Here, we reveal the extended and contracted atomic structures of an intact contractile-tailed phage (φCD508) that binds to and penetrates the protective S-layer of the Gram-positive human pathogen Clostridioides difficile. The virion can be divided into five distinct regions: the head, neck, tail, baseplate, and needle. Structures of purified φCD508 virions in both extended and contracted conformations were determined by single-particle EM of frozen-hydrated samples; the resolution ranged from 2.6 to 4.0 Å for the extended phage, and 2.9 to 4.2 Å for the contracted form.

The tail is attached to the neck and made up of a stack of 57 nested hexameric tail protein rings, with an inner ring of the tail tube protein gp56 and an outer ring of the tail sheath protein gp55. Each ring is offset from those above and below such that the extended tail assembly can be described as a six-stranded helix, with a twist of 19°, a rise of 39 Å, and an outer diameter of 230 Å. However, a notable feature is that the tail is considerably longer (225 nm) than those of other phages whose structures have been described. In the extended state (left), the sheath forms extensive interactions between the sheath and the tail tube. The main tail tube protein, gp56, has the conserved fold seen in other Caudoviricetes tail tubes. However, gp56 lacks both the ɑ-loop and the N-loop seen in other myovirus tail tube proteins, as well as the C-terminal loops seen in siphovirus tail tube proteins. The gp55 tail sheath protein is made up of three domains. The tail tube–proximal domain I contains a loop consisting of residues 368–378, which is twice as long in φCD508 than in the sheath domains of pyocins, AFP, and PVC (six residues and three residues, respectively). Domains I and II reside in strong density, but domain III lacks density because of flexibility in the region.

>MATGTWNEKERKEIPGFYNRFKTQAEKSTNTGLKGRLAMPIRANWGDVGKVVTIKNDLRQLKNLFGDDMNYSAFKLGKLALLGNVKELLLYRLVDGNQKKGTLTLKDTTENSAKDVIKLETKYPTARNFNVTIKSNLVDSDKKDFIFFENTKQLFSSSIKGTIDEIVLEINSNLDNEYVIATKVADSDTILANVVNQALEGGNDGCTSITNESYLKALEEFERYSFDSFVLDGVADEALQETTKAWVAKNKELGKDILLFLGGKTEDNIKQINDKSKSFNDENIVNVGSSAYYENIKYTPSEVAVYIAALSVSKGITGSICNAKTIFEEVEPRLSQSEVKECLKSGTLVLDFDDGDVIIVDDVNTFKKYVDDKNEAMGYISNIMFINTINKDTSLKRKEFVGKIFNDATGQTTVICALKKYFEELMSQGIISEFNVDIDTELQATAKADEFYWKWDAVKVDVMKKIYGTGYLG[18x];>[18x]MYNDDYIEEASFLNGSDVVILIDGVEELYMEEIKADFEQDEQSIKLLGCQNEISRVGTTKGSFSLNGYKTDSKFAKLGFRSFEIIYNLSNSETLGYESIRLKNCRLKKLPLINSKAGEIVKIEVEGSFRGYDLLNEL>MHHHHHHFSGLVPRGSHMESLRDGMLVGLGNPLLDISAVVEKDLLNKYDMQPNNAILAEEKHMPMYQELIEKYQAEYIAGGSVQNSLRVAQWILQRPRTAIFFGCVGQDEYARILEERATSNGVNVQYQRSATSPTGTCAVLVTGTQRSLCANLAAANDFTPEHLRSDGNRAYLQGAQFFYVSGFFFTVSFESALSVAKEAAATGRMFMMNLSAPFVPQFYKNNLEEIFPYVDVLFGNETEAIALAKEFNYGTEDLREIGKRIAALPKENGKRKRIVIITQGSDPVLLIEAGTDNVREFPVQKLAPEQMVDTNGAGDAFVGGFLAQLLQSRTVDVCIKCGIWAA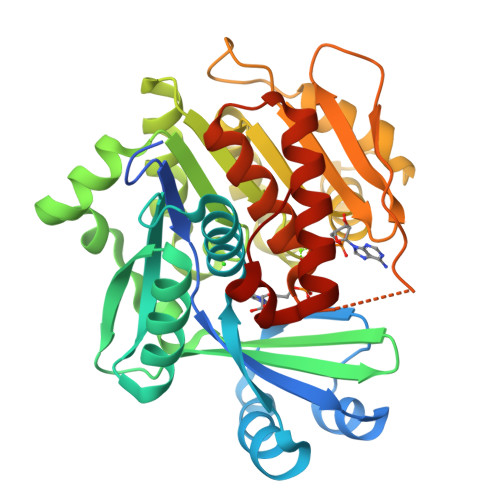REIIQRSGCTFEGEPSFCADN[3x]>MGSSHHHHHHSSGRENLYFQG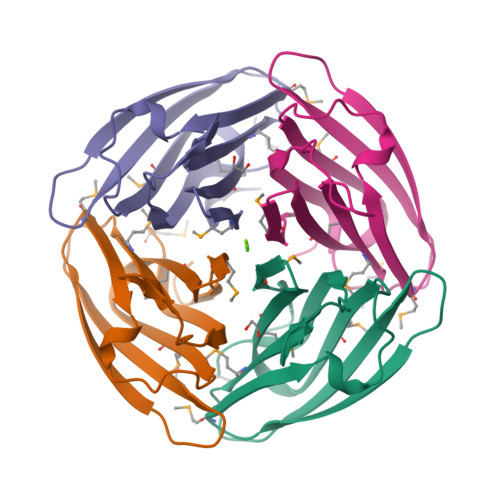HMNGARKWFFPDGYIPNGKRGYLVSHESLCIMNTGDETAKIRITFLFEDSKPVVHEVEISPMKSLHLRLDKLGIPKCKPYSIMAESNVPVVMQLSRLDVGKNHYTLMTTIGYWEEGS[4x]>[2x]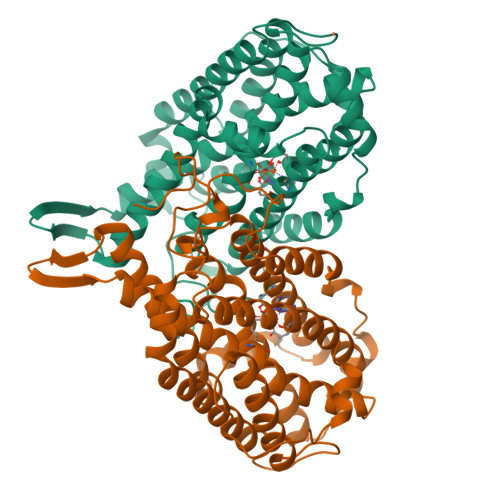AYTTFSQTKNDQLKEPMFFGQPVNVARYDQQKYDIFEKLIEKQLSFFWRPEEVDVSRDRIDYQALPEHEKHIFISNLKYQTLLDSIQGRSPNVALLPLISIPELETWVETWAFSETIHSRSFTHIIRNIVNDPSVVFDDIVTNEQIQKRAEGISSYYDELIEMTSYWHLLGEGTHTVNGKTVTVSLRELKKKLYLCLMSVNALEAIRFYVSFACSFAFAERELMEGNAKIIRLIARDEALHLTGTQHMLNLLRSGADDPEMAEIAEECKQECYDLFVQAAQQEKDWADYLFRDGSMIGLNKDILCQYVEYITNIRMQAVGLDLPFQTRSNPIPWINTWLV> SELRTLPVLPLRDIVVFPHMVVPLFVGRDKSVRALEEVMRGDKQILLVTQKNSADDDPAPGDIFEVGVLATVLQLLKLPDGTVKVLVEGKARAAVVSFTDQESYYEAQIGEVSEDDGAGPEAEALSRAVVEQFENYVKLNKKVPPEALASIPQIAEPGKLADSIAAHLSVKIGDKQ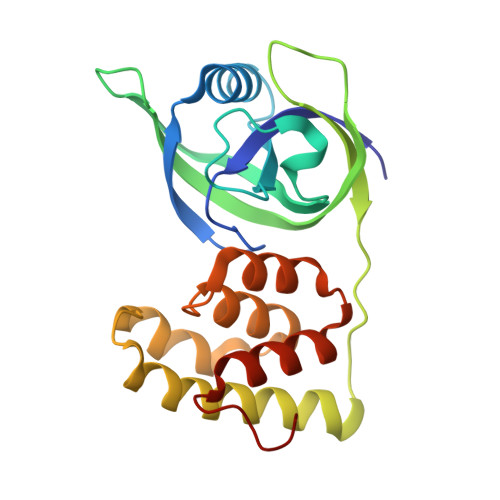NLLEIFDVVKRLEKVFALMEGEISVLQVEK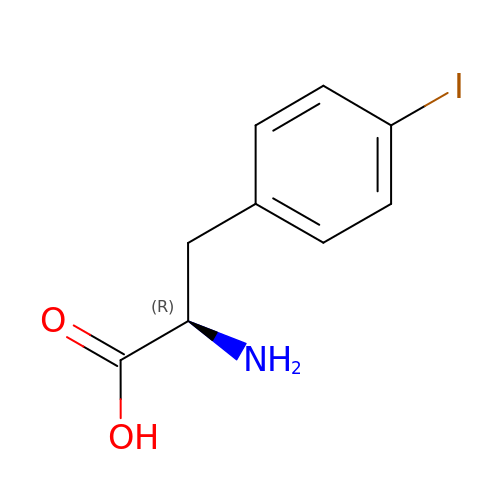P-IODO-D-PHENYLALANINE | C9 H10 I N O2 | PZNQZSRPDOEBMS-MRVPVSSYSA-N>GAMGRLNQRNINELKIFFEKAKYYSIKLDAIYNEYTEAYNDIMTYSEVNNVTDSDKSKVNQAISILKKDNKIVNKFKELEKIIEEYKPIFLSKLIDDFAIELDQAVDNDVSNARHVADSYKKLRKSVVLAYIESFDVISSKFVDSKFVEASKKFVNKAKEFVEENDLIALECIVKT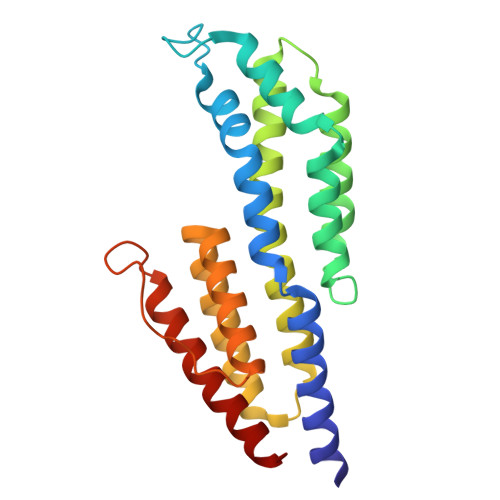IGDMVNDREINSRSRYDNFYKKEADFLGAAVELEGAYKAIKQTLL[2x]>[2x]MDHLPIFCQLRDRDCLIVGGGDVAERKARLLLEAGARLTVNALTFIPQFTVWANEGMLTLVEGPFDETLLDSCWLAIAATDDDTVNQRVSDAAESRRIFCNVVDAPKAASFIMPSIIDRSPLMVAVSAGGTSPVLARLLREKLESLLPQHLGQVARYAGQLRARVKKQFATMGERRRFWEKFFVNDRLAQSLANADEKAVNATTERLFSEPLDHRGEVVLVGAGPGDAGLLTLKGLQQIQQADIVVYDRLVSDDIMNLVARDADRVFVGKRAGYHCVPQEEINQILLREAQKGKRVVRLKGGDPFIFGRGGEELETLCHAGIPFSVVPGITAASGCSAYSGIPLTHRDYAQSVRLVTGHLKTGGELDWENLAAEKQTLVFYMGLNQAATIQEKLIAFGMQADMPVALVENGTSVKQRVVHGVLTQLGELAQQVESPALIIVGRVVALRDKLNWFSNH

Siroheme is the modified isobacteriochlorin tetrapyrrole used by siroheme-dependent sulfite and nitrite reductases (SiR/NiRs) in catalyzing the six-electron reduction of sulfite to sulfide or nitrite to ammonia. CysG is encoded by a gene fusion between a C-terminal SUMT (CysGA) and an N-terminal bifunctional dehydrogenase/ferrochelatase (CysGB). The N-terminal enzyme module, CysGB, is a three-domain bifunctional dehydrogenase/ATP-independent class III ferrochelatase12 that performs the final two steps of siroheme biosynthesis. The C-terminal enzyme module, CysGA, is homologous to a well-studied class of SAM-dependent uro’gen III methyltransferases (SUMTs) that catalyzes the methylations to generate precorrin-210,13.

R260, which binds ring C C12 acetyl, and R261, which does not directly interact with carboxylate but contributes to the positively charged pocket that captures ring B, are part of the CysGA SUMT module. To test whether or not their contributions are essential for tetrapyrrole binding, we individually altered each to an alanine and tested the variants’ activities for dehydrogenase or chelatase activity. Both the R260A and R261A variants complement a cysG deficiency in E. coli grown on minimal media where SO42− is the sole sulfur source. Interestingly, the culture expressing R260A, but not R261A, showed signs of precorrin-2 buildup in its pink fluorescence. Activity assays showed that the R260A variant is deficient for dehydrogenase activity and ~100-fold less active as a chelatase. Non-enzymatic oxidation of precorrin-2 is sufficient to support complementation of a dehydrogenase-deficient but chelatase-active enzyme, explaining why R260A complemented despite deficiency for dehydrogenase activity. We next determined the X-ray crystal structures of the variants to test whether these alterations changed the relationship between the enzyme modules or their overall structure. Both R260A and R261A structures are similar to CysG and have a low root-mean-square deviation (RMSD) when aligned against Met8p14. R260 directly interacts with the ring C carboxylates, but removing the large side chain does not substantially alter CysG’s structure despite its participation in forming the active site. The R260A variant was deficient for dehydrogenase activity and significantly reduced for metal insertion.>G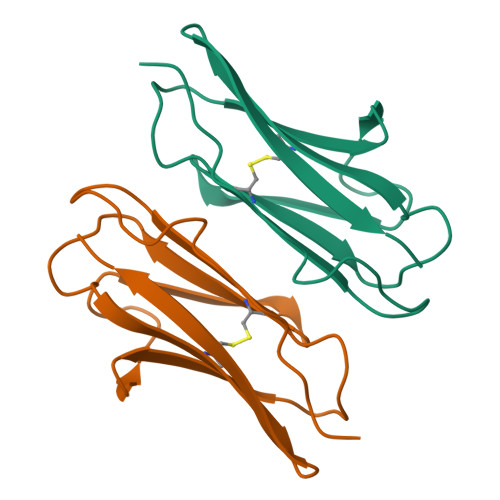ASGSVPPQVLPFSFGESAADVGDIASANCVVPKGDLPLEIRWSLNSAPIVNGENGFTLVRLNKRTSLLNIDSLNAFHRGVYKCIATNPAGTSEYVAELQVN[4x]>GTGDGSMPATVAELQAEIAAWIHPLNPDRRPGGTIAKLLEEIGELIASDRAHDPLEVADVLILALDLATLLGVDVTE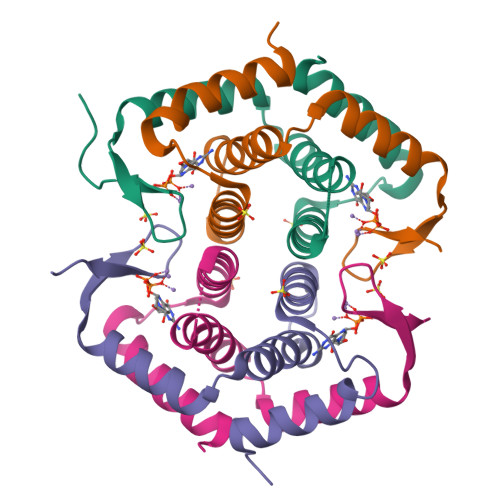AIRAKLAINRARSWARADNGAMRHIPGSDTPSFP[4x]>[4x]MVKIPKSHPRYWSLYYREKIIEGMEKGMTAKAGLIAHGRGEAFDYLIGERTIEPAERAMRAAVAKLLLAENPVVSVNGNVAALVPKETIELARALNAKLEINLFYRTEDRVKAIAEELRKYDPEIELLGINPTKRIPGLEHERGKVDENGIWKADVVVVPLEDGDRTEALVRMGKFVITIDLNPLSRSARMADITIVDNIVRAYPRMTELAREMKDYSRGELI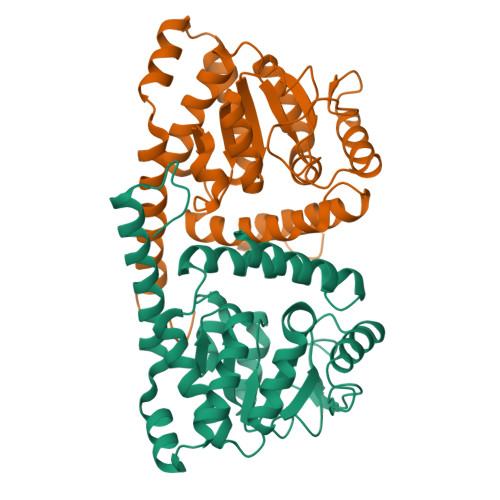RIIEEYDNGKTLNDVLLHIRDRLTKLAEGGIWRKKQLD> MATGQDRVVALVDMDCFFVQVEQRQNPHLRNKPCAVVQYKSWKGGGIIAVSYEARAFGVTRSMW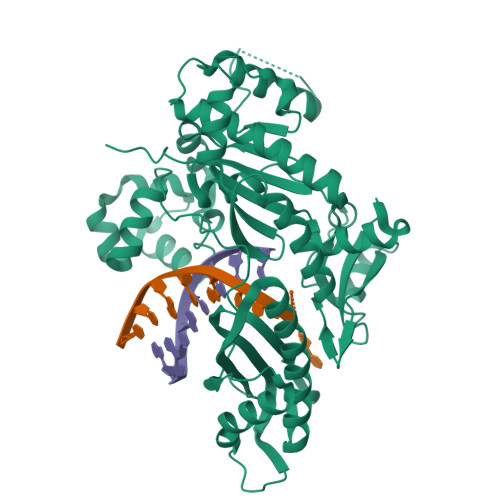ADDAKKLCPDLLLAQVRESRGKANLTKYREASVEVMEIMSRFAVIERASIDEAYVDLTSAVQERLQKLQGQPISADLLPSTYIEGLPQGPTTAEETVQKEGMRKQGLFQWLDSLQIDNLTSPDLQLTVGAVIVEEMRAAIERETGFQCSAGISHNKVLAKLACGLNKPNRQTLVSHGSVPQLFSQMPIRKIRSLGGKLGASVIEILGIEYMGELTQFTESQLQSHFGEKNGSWLYAMCRGIEHDPVKPRQLPKTIGCSKNFPGKTALATREQVQWWLLQLAQELEERLTKDRNDNDRVATQLVVSIRVQGDKRLSSLRRCCALTRYDAHKMSHDAFTVIKNCNTSGIQTEWSPPLTMLFLCATKFSAS>[26x]MELFDENYYAKAVANIIGEVKDPIMYKWFSPDQIEDVDLQMGYQKTVKWDAFLNANPTTIANEVNTISTIGFSSEVVRLNYLKLQYKFRHLKQTSEKFYTSDSYIGDINNNLLPFAQAYKLASSEIIKLINHFVLTGTVSIQKDGKNQKRLLPNMYGLLNMPEQIKEEVASGDKDKMDKIFEKIEAGLSKLELGDEFSTPMMVIVDPATSLKLVKPYAAAQGAASSCEKWEDVLIQTIKAINNREDVYIETSNLLKHKILIYPLNSELIKFKPSKYMLPTPNEQVDKDSTDVAHSYIDFVLGGLLATRKTILQVNIKQS;>[15x]MSDITKIKQEFDKKVAEIQALMKNPQQDSGLLSNSIDFRDQNLIFSNSGGVCTSSKDKIENYPAKGYPYKRGVKLSFGDGTTELEVEAGGGDDLYGVCSDIDEFSGMATVIPITNNFTGYLTLKKDGQNGVNPGDKLNFNQHGELEKVTGAQKSVNAIALSKAHKLTEDLFIVLASVFGNRAIKG;>MG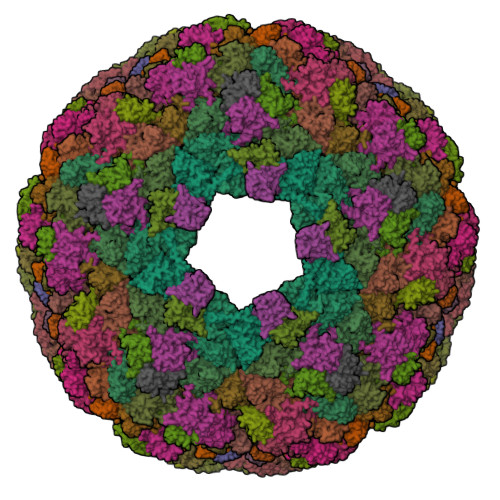DTTQLVKEYQEKRSKLEKFMKNPQHDASLLSNSNEFRDKNVEFFASGGTRTSKFDKLENHPFLGYPYKRGVKRVIQEAQDNQSHYEPHVEAGGGEDLYGICIDIDEFSKTATIVPITNNFEGYLVAKDSTVKVKDKLIFNKDGALEKVTGAPNKATINATALTDAKQISNEVYLVKVAVFGNKAMSRN[7x];>MTEKEEKEDLQAQDKEEQQIKADTKVISVQEFEEYMRFKEQANSKSKETSRDLSINERITKELAEVEERERIEKQLLLEAERINEIDTLAKAHLSNHFNKEVLLAKGYTLKDIMQAQRRELVRKFVPIEQIKAIAKVSDISHIDGEILEQLVSLAKVNIKLRKNASSSSSSVDSIKGNIAIKSEERASLLDSNFVPINFTEFVQAISNTYKQRRIQFYENLKRHKRTSIA[26x];> MALKGNMQVENLEAVEDPQVDLGAQVSAAPRAKRQARQAEDVQGEDPYLESISELDDVLLKFKKYSKSMSSIENKVFSSSSGCFKSKNERVDAYSFACSSYTDKIEEYLYDPANSFPYKRGVKLVPKENSIYVEVGADTDMYGICVDVCEFSCTAYVLPITNNFEGYLVTRNPSIKIGEILDINNNGVIIKAGGGPPTAINIYALSDSFTINFAPEDGNQDQNRYPRQEYSINLIKVAIFGNRGLEKTVNPDGG>[3x]MVRKGEKKLAKPATTKAANPQPRRRANNRRRSNRTDAPVSKASTVTGFGRGTNDVHLSGMSRISQAVLPAGTGTDGYVVVDATIVPDLLPRLGHAARIFQRYAVETLEFEIQPMCPANTGGGYVAGFLPDPTDNDHTFDALQATRGAVVAKWWESRTVRPQYTRTLLWTSSGKEQRLTSPGRLILLCVGNNTDVVNVSVLCRWSVRLSVPSLETPEETTAPIMTQGSLYNDSLSTNDFKSILLGSTPLDIAPDGAVFQLDRPLSIDYSLGTGDVDRAVYWHLKKFAGNAGTPAGWFRWGIWDNFNKTFTDGVAYYSDEQPRQILLPVGTVCTRVDSEN

Betanodaviruses are small, spherical, non-enveloped viruses with a bipartite single-stranded (+) RNA genome encapsulated by 180 molecules of a single self-assembly capsid protein (CP). Piscine nodaviruses, the causal agents of viral nervous necrosis (VNN) or viral encephalopathy and retinopathy (VER), are members of the BetanodavirusNodaviridae family. VLP are well-structured particles with high similarity to native virions and they can assemble spontaneously from single (i.e. betanodavirus CP) or multiple structural proteins under specific conditions.

Firstly, the 3D structure of native OGNNV VLP (RBS) at 3.9 Å resolution was determined. The 3D structure of RBS reveals that RBS has a capsid with 30 nm in diameter with T = 3 icosahedral symmetry. Outside of the surface of the capsid, there are 60 protrusions located at the top of the center of each asymmetry unit, and with the protrusions, the diameter of the whole RBS enlarges to be around 38 nm. There are three chemical identical subunits with slight conformational variations in the spatial location, VPa, VPb and VPc, in each asymmetric unit. We could only identify the densities of residues 52–220 of VPa and VPb. While for VPc, we could detect the densities of 17 more amino acid residues at the N-terminal. These 17 amino acids compose a loop from the two fold axis and cross the VPb, then form a trident structure with another two N-terminus of the VPc at the three fold. Accordingly, we separate CP into three independent domains: the N-terminal domain (N domain) (residues 1–50), the Shell domain (S domain) (residues 51–220) and the Protrusion domain (P domain) (221–338). The S domain is mainly composed of a canonical jelly-roll, and a β-barrel fold containing eight antiparallel β-strands. Between S and P domains, there is a high flexible linker loop composed of residues 210–220 functioning as a connection.> MDIIL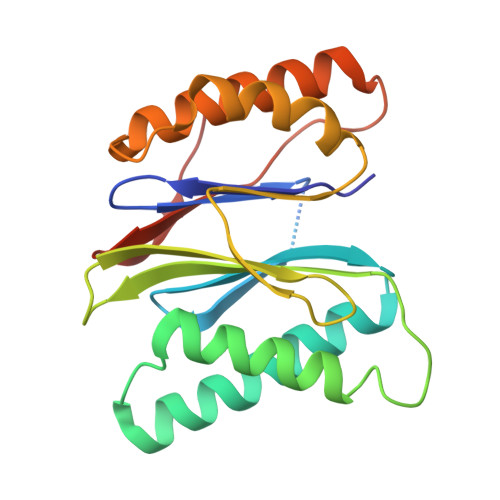GIRVQDSVILASSKAVTRGISVLKDSDDKTRQLSPHTLMSFAGEAGDTVQFAEYIQANIQLYSIREDYELSPQAVSSFVRQELAKSIRSRRPYQVNVLIGGYDKKKNKPELYQIDYLGTKVELPYGAHGYSGFYTFSLLDHHYRPDMTTEEGLDLLKLCVQELEKRMPMDFKGVIVKIVDKDGIRQVDDFQAQ>[2x]MNTMLFSPYTIRGLTLKNRIVMSPMCMYSCDTKDGAVRTWHKIHYPARAVGQVGLIIVEATGVTPQGRISERDLGIWSDDHIAGLRELVGLVKEHGAAIGIQLAHAGRKSQVPGEIIAPSAVPFDDSSPTPKEMTKADIEETVQAFQN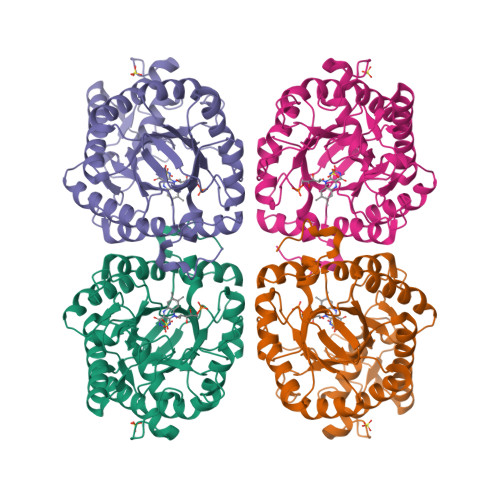GARRAKEAGFDVIEIHAAHGYLINEFLSPLSNRRQDEYGGSPENRYRFLGEVIDAVREVWDGPLFVRISASDYHPDGLTAKDYVPYAKRMKEQGVDLVDVSSGAIVPARMNVYPGYQVPFAELIRREADIPTGAVGLITSGWQAEEILQNGRADLVFLGRELLRNPYWPYAAARELGAKISAPVQYERGWRF> GAMGSAVSESQLKKMVSKYKYRDLTVRE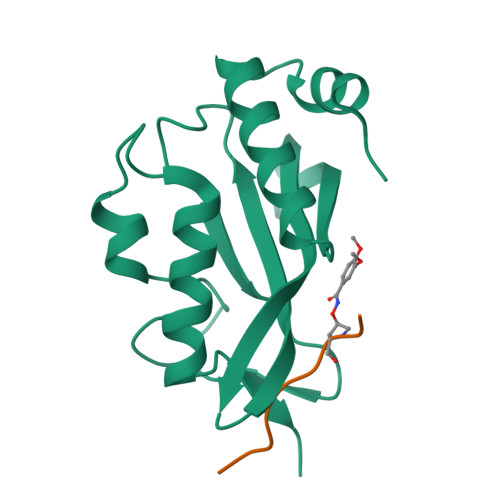TVNVITLYKDLKPVLDSYGGSRELMNLTGTIPVPYRGNTYNIPICLWLLDTYPYNPPICFVKPTSSMTIKTGKHVDANGKIYLPYLHEWKHPQSDLLGLIQVMIVVFGDEPPVFSRP The Pden_5119 protein oxidizes NADH with oxygen under mediation by the bound flavin mononucleotide (FMN) and may be involved in the maintenance of the cellular redox pool. The findings so far indicate that the Pden_5119 protein shares functional properties with both flavin reductases, which use flavin as a dissociable cosubstrate, and flavoprotein oxidases, which contain flavin as a permanently bound cofactor. It follows a sequentially ordered mechanism where FMN binds before NADH and the binary complex enzyme-reduced flavin formed after the hydride transfer persists for a long enough time to be oxidized by molecular oxygen. Structural and kinetic data suggest that His-117 plays a role in the binding and positioning of the isoalloxazine ring of FMN, Lys-82 fixes the nicotinamide ring of NADH to support the proS-hydride transfer, and Arg-116 with its positive charge promotes the reaction between dioxygen and reduced flavin.

In order to understand the structural basis for Pden_5119 catalysis, single crystals of this enzyme were prepared and used to collect diffraction data (resolution range 48.75–3.1 Å). The monomer takes a flavodoxin-like fold with a central β sheet made up of five parallel strands in the order 21345 which is sandwiched between helices 1 and 5 on one side and helices 2, 3, and 4 on the other side. The oligomeric state in solution was analyzed by means of small-angle X-ray scattering (SAXS). Ab initio modeling using the SAXS data obtained at a protein concentration of 1.5 mg·mL−1 (73 μM in monomer) yielded an envelope that has space for the dimer. Therefore, we can conclude that the dimer represents the major species in the solution. Despite co-crystallization and soaking trials, we could not obtain crystals of Pden_5119 containing bound FMN. The FMN molecule position was therefore predicted by in silico docking analysis. Further inspection of the isoalloxazine environment implicated three amino acid residues, His-117, Lys-82, and Arg-116, as potentially involved in catalysis. The imidazole ring of His-117 is positioned to form a hydrogen bond with the N3 nitrogen of FMN similar to the case for homologous His-112 and His-116 residues in SsuE and EmoB.

>MPGPRIVAFAGSWSRPSKTRSLVEEAARRAVARFGGSAHVFDIADLGPDFGSLRQPQDGPHTRHLDAFLAADALIVASPVYKGSYTGLFKHFIDLIEPVALVGKPVLLAATGGGDRHALVIEHQLRPVFGFFEAHTLATGLYVSASDFGPDGLASEAASTRLDRAVAQFAAHLSRHDAAPLLAVGLEHHHHHH[20x]>[4x]PTTKVKLECNPTARIYRKHFLGKEHFNYYSLDTALGHLVFSLKYDVIGDQEHLRLLLRTKCRTYHDVIPISCLTEF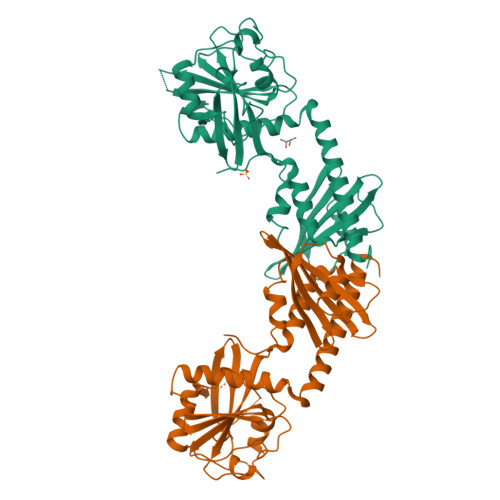PNVVQMAKLVCEDVNVDRFYPVLYPKASRLIVTFDEHVISNNFKFGVIYQKLGQTSEEELFSTNEESPAFVEFLEFLGQKVKLQDFKGFRGGLDVTHGQTGTESVYCNFRNKEIMFHVSTKLPYTEGDAQQLQRKRHIGNDIVAVVFQDENTPFVPDMIASNFLHAYVVVQAEGGGPDGPLYKVSVTARDDVPFFGPPLPDPAVFRKGPEFQEFLLTKLINAEYACYKAEKFAKLEERTRAALLETLYEELHIHSQSMMGLGGDE> MSDSHHKPVWDRTHHAKMATGIGDPQCFKGMAGKSKFNVGDRVRIKDLPDLFYTRTMTYTRGATGTIVRLVYESPAAEDEAFGNEENVEWFYSIVFAQKDLWPEYSDTFANDTLETEIPERYL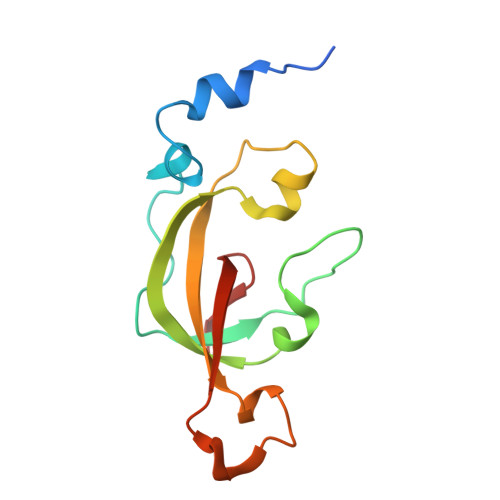EKA> MAANMYRVGDYVYFENSSSNPYLIRRIEELNKTANGNVEAKVVCFYRRRDISSTLIALADKHATLSVCYKAGPGADNGEEGEIEEEMENPEMVDLPEKLKHQLRHRELFLSRQLESLPATHIRGKCSVTLLNETESLKSYLEREDFFFYSLVYDPQQKTLLADKGEIRVGNRYQADITDLLKEGEEDGRDQSRLETQVWEAHNPLTDKQIDQFLVVARSVGTFARALDCSSSVRQPSLHMSAAAASRDITLFHAMDTLHKNIYDISKAISALVPQGGPVLCRDEMEEWSASEANLFEEALEKYGKDFTDIQQDFLPWKSLTSIIEYYYMWKTTDRYVQQKRLKAAEAESKLKQVYIPNYNKPNPNQISVNNVKAGVVNGTGAPGQSPGAGRACESCYTTQSYQWYSWGPPNMQCRLCASCWTYWKKYGGLKMPTRLDGERPGPNRSNMSPHGLPARSSGSPKFAMKTRQAFYL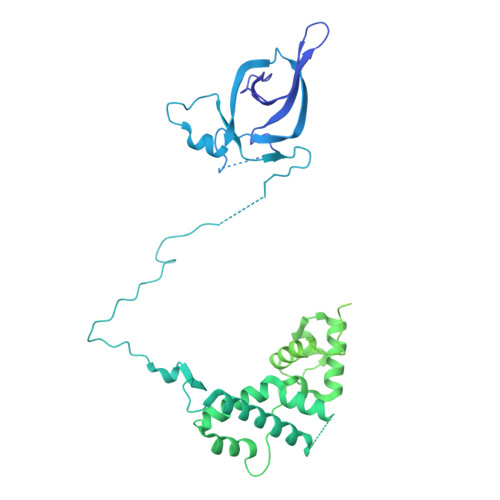HTTKLTRIARRLCREILRPWHAARHPYLPINSAAIKAECTARLPEASQSPLVLKQAVRKPLEAVLRYLETHPRPPKPDPVKSVSSVLSSLTPAKVAPVINNGSPTILGKRSYEQHNGVDGNMKKRLLMPSRGLANHGQARHMGPSRNLLLNGKSYPTKVRLIRGGSLPPVKRRRMNWIDAPDDVFYMATEETRKIRKLLSSSETKRAARRPYKPIALRQSQALPPRPPPPAPVNDEPIVIED>[4x]MLKGKVAVVTGSTSGIGLGIATALAAQGADIVLNGFGDAAEIEKVRAGLAAQHGVKVLYDGADLSKGEAVRGLVDNAVRQMGRIDILVNNAGIQHTALIEDFPTEKWDAILALNLSAVFHGTAAALPHMKKQGFGRIINIASAHGLVASANKSAYVAAKHGVVGFTKVTALETAGQGITANAICPGWVRAPLVEKQ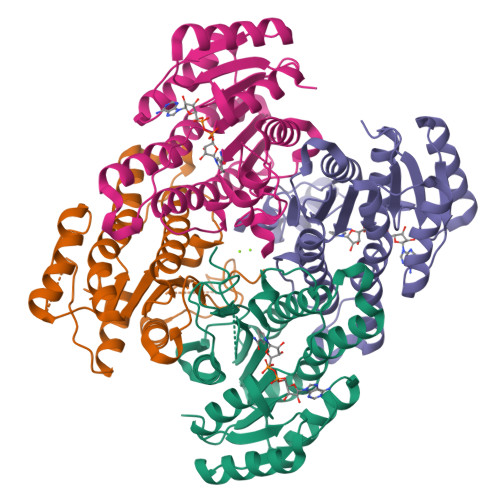ISALAEKNGVDQETAARELLSEKQPSLQFVTPEQLGGTAVFLASDAAAQITGTTVSVDGGWTAR Collagen prolyl 4‐hydroxylase (C‐P4H) catalyzes the 4‐hydroxylation of Y‐prolines of the XYG‐repeat of procollagen. The α‐subunit provides the N‐terminal dimerization domain, the middle peptide‐substrate–binding (PSB) domain, and the C‐terminal catalytic (CAT) domain. There are three isoforms of the α‐subunit, complexed with a β‐subunit that is protein disulfide isomerase, forming C‐P4H I‐III. The PSB domain of the α‐subunit binds proline‐rich peptides, but its function with respect to the prolyl hydroxylation mechanism is unknown.

An extended mode of binding of proline‐rich peptides (PPII, polyproline type‐II, conformation) to the PSB‐I domain has previously been reported for the PPG‐PPG‐PPG and P9 peptides. Crystal structures now show that peptides with the motif PxGP (PPG‐PRG‐PPG, PPG‐PAG‐PPG) (where x, at Y‐position 5, is not a proline) bind to the PSB‐I domain differently, more deeply, in the peptide‐binding groove. The latter mode of binding has previously been reported for structures of the PSB‐II domain complexed with these PxGP‐peptides. Calorimetric binding studies show that the affinities of these peptides are lower for PSB‐I than for PSB‐II, with, respectively, K D values of about 70 μM for PSB‐I and 20 μM for PSB‐II.

>[2x]MSFLTAEDCFELGKVAYTEADYYHTELWMEQALRQLDEGEISTIDKVSVLDYLSYAVYQQGDLDKALLLTKKLLELDPEHQRANGNLKYFEYIMAKELEHHHHHH;>PPGPAGPPG[2x]>GPRARDLGVPFEGTPGALNAITDVAGVEVGHTTVISGDGAMVIGKGPYRTGVTIIHPLGKTSLDGVAAGRAVINGTGEWTGMHLVDEVGQFLGPIALTGTGNVGLVHQSMMDWSVGKVPEEALFSRLLPVVAETLDNRLNDVFGHGLTRDHVFAALDGAKGGPVAEGNVGGGTGMIAYTFKGGIGTSSRVVSAGDTRYTVGVLVQANHGDRNDLRIAGVQIGKEIKGAWPEVNGIVAAGPDAGKPQDKNALLIVIATDAPLMPHQLERMARRAALGVGRNGSTAGALSGEFALAFSTSHVIPLGGKPRLPAIINDTDSETMNALFRGVVQATEEALVNQLVASETMTGANNAKVYGIPHDQLARIMKA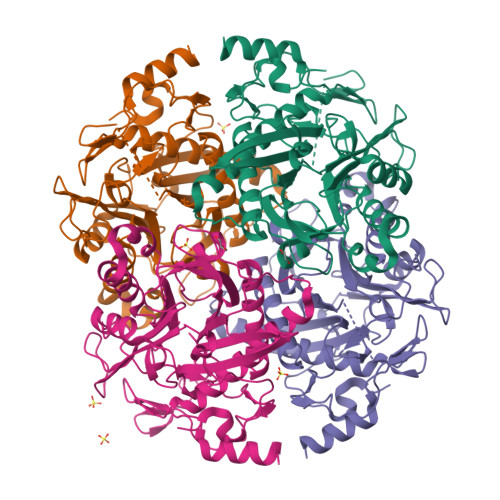RFPRR[4x]>MVRSFIYEPFQIPSGSMMPTLLIGDFILVEKFAYGIKDPIYQKTLIETGHPKRGDIVVFKYPEDPKLDYIKRAVGLPGDKVTYDPVSKELTIQPGCSSGQACENALPVTYSNVEPSDFVQTFSRRNGGEATSGFFEVPKNETKENGIRLSERKETLGDVTHRILTVPIAQDQVGMYYQQPGQQLATWIVP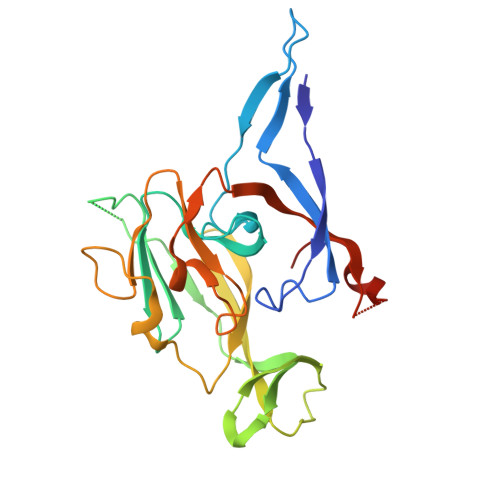PGQYFMMGDNRDNSADSRYWGFVPEANLVGRATAIWMSFDKQEGEWPTGLRLSRIGGIH[4x]>NLYFQHMRHFARTHAIGQIVPGKVTKLVPFGAFVRVEEGIEGLVHISELAERHVEVPDQVVAVGDDAMVKVIDIDLERRRISLSLKQANEDYTEEFD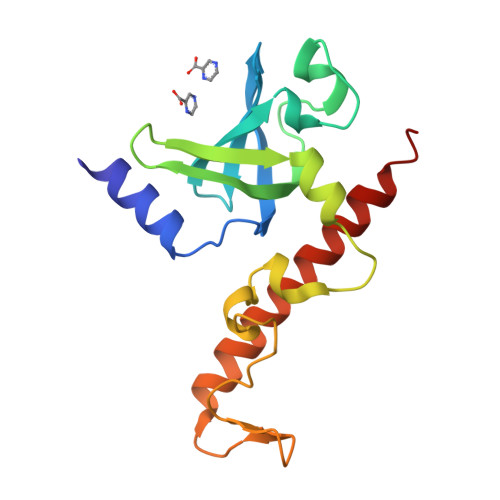PAKYGMADSYDEQGNYIFPEGFDAETNEWLEGFEKQRAEWEARYAEAERRHKMHTAQMEKFAAA[2x]> MEKVFYVTTPIYYVNAEPHLGHAYTTVVADFLARWHRLDGYRTFFLTGTDEHGETVYRAAQAAGEDPKAFVDRVSGRFKRAWDLLGIAYDDFIRTTEERHKKVVQLVLKKVYEAGDIYYGEYEGLYCVSCERFYTEKELVEGLCPIHGRPVERRKEGNYFFRMEKYRPWLQEYIQENPDLIRPEGYRNEVLAMLAEPIGDLSISRPKSRVPWGIPLPWDENHVTAVWFDALLNYVSALDYPEGEAYRTFWPHAWHLIGKDILKPHAVFWPTMLKAAGIPMYRHLNVGGFLLGPDGRKMSKTLGNVVDPFALLEKYGRDALRYYLLREIPYGQDTPVSEEALRTRYEADLADDLGNLVQRTRAMLFRFAEGRIPEPVAGEELAEGTGLAGRLRPLVRELKFHVALEEAMAYVKALNRYINEKKPWELFKKEPEEARAVLYRVVEGLRIASILLTPAMPDKMAELRRALGLKEEVRLEEAERW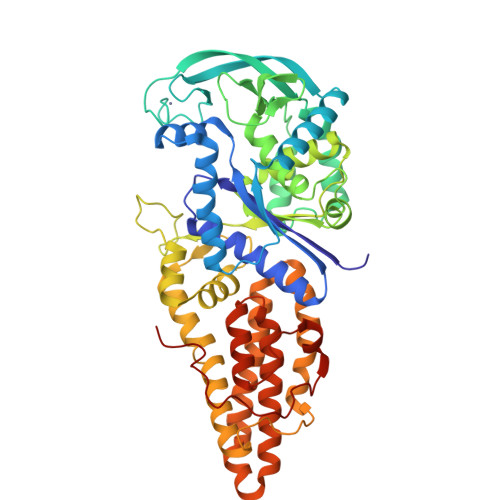GLAEPRPIPEEAPVLFPKKEA>MSLDFHGVFPYLVSPVDAEGRVRADVMGRLCDDLIQAGVHGLTPLGSTGEFAYLGTAQREAVVRATIEAAQRRVPVVAGVASTSVADAVAQAKLYEKLGADGILAILEAYFPLKDAQIESYFRAIADAVEIPVVIYTNPQFQRSDLTLDVIARLAEHPRIRYIKDASTNTGRLLSIINRCGDALQVFSASAHIPAAVMLIGGVGWMAGPACIAPRQSVALYELCKAQRWDEALMLQRKLWRVNEAFAKFNLAACIKAGLALQGYDVGDPI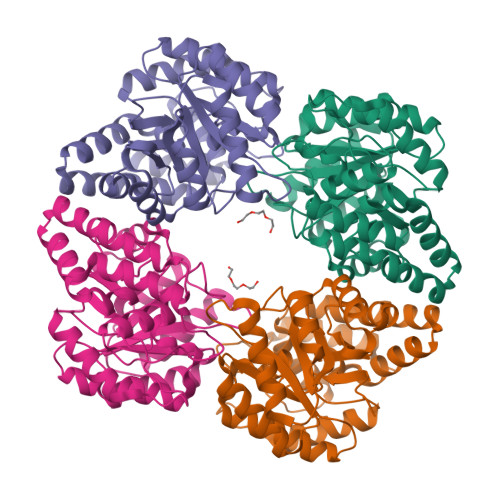PPQAALTAEERKAVEKVLAEIAEGHHHHHH[4x]>[2x]MRVPEKYSTLPAEDRSVHIVNICAIEDLGYLPSEGTLLNSLSVDPDAECKYGLYFRDGKRKVDYILVYHHKRASGSRTLARRGLQNDMVLGTRSVRQDQPLPGKGSPVDAGSP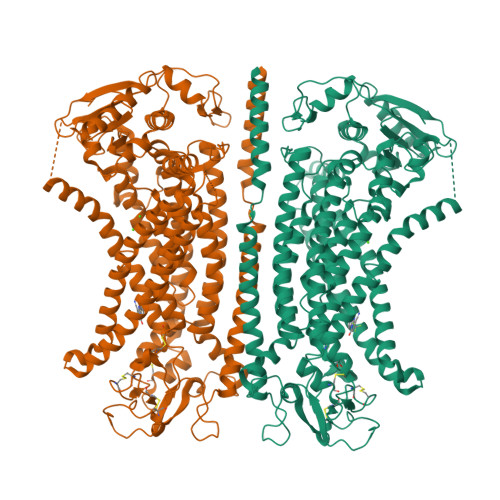EVPMDYHEDDKRFRREEYEGNLLEAGLELENDEDTKIHGVGFVKIHAPWHVLCREAEFLKLKMPTKKVYHISETRGLLKTINSVLQKITDPIQPKVAEHRPQTTKRLSYPFSREKQHLFDLTDRDSFFDSKTRSTIVYEILKRTTCTKAKYSMGITSLLANGVYSAAYPLHDGDYEGDNVEFNDRKLLYEEWASYGVFYKYQPIDLVRKYFGEKVGLYFAWLGAYTQMLIPASIVGVIVFLYGCATVDENIPSMEMCDQRYNITMCPLCDKTCSYWKMSSACATARASHLFDNPATVFFSVFMALWAATFMEHWKRKQMRLNYRWDLTGFEEEEEAVKDHPRAEYEARVLEKSLRKESRNKETDKVKLTWRDRFPAYFTNLVSIIFMIAVTFAIVLGVIIYRISTAAALAMNSSPSVRSNIRVTVTATAVIINLVVIILLDEVYGCIARWLTKIEVPKTEKSFEERLTFKAFLLKFVNSYTPIFYVAFFKGRFVGRPGDYVYIFRSFRMEECAPGGCLMELCIQLSIIMLGKQLIQNNLFEIGIPKMKKFIRYLKLRRQSPSDREEYVKRKQRYEVDFNLEPFAGLTPEYMEMIIQFGFVTLFVASFPLAPLFALLNNIIEIRLDAKKFVTELRRPVAIRAKDIGIWYNILRGVGKLAVIINAFVISFTSDFIPRLVYLYMYSQNGTMHGFVNHTLSSFNVSDFQNGTAPNDPLDLGYEVQICRYKDYREPPWSEHKYDISKDFWAVLAARLAFVIVFQNLVMFMSDFVDWVIPDIPKDISQQIHKEKVLMVELFMREEQGKQQLLDTWMEKEKPRDVPCNNHSPTTHPEAGDGSPVPSYEYHGDAL>[4x]MKLDDLNLFRLVVENGSYTSTSKKTMIPVATITRRIQALEDSLNLRLLNRHARKLTLTEAGERFYKDCSPLLERLASMTEEITDECRGASGRIRISAPSELTKRMMMPMFNAFMEKYPDIHIELMMSNQADDLDPTEWDVIFRVGPQRDSSLIARKIGEVKDILVASPQYLSSHPQPTHAEELHQHQLL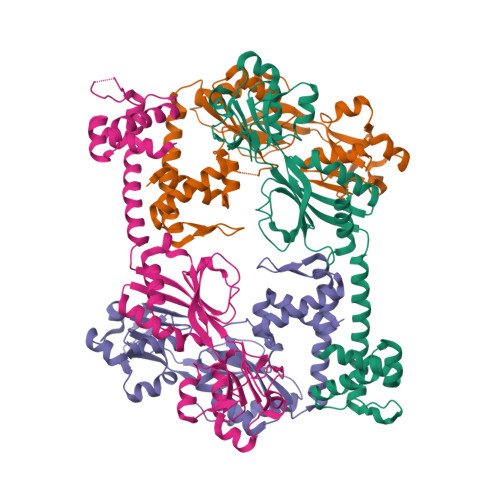KGYPLLKWQLTNSQGETVVNSDRGRFQASALNVVRSACSEGLGITLMPDVMLREFLEDGSLVQVLSDWSSNPRDIYMLYNHKDHQPEKVRLFIDFVIGYHLQ>DANLTPDIRADIHAELVRLSFMPTRSESERYAIADRALAQYAALEILWHDNPDRTAQYQRIQVDHLGALLTRDRYKDVISHYQRLKKTGQIIPPWGQYWVASAYLKDHQPKKAQSIMTELFYHKETIAPDLSDEEL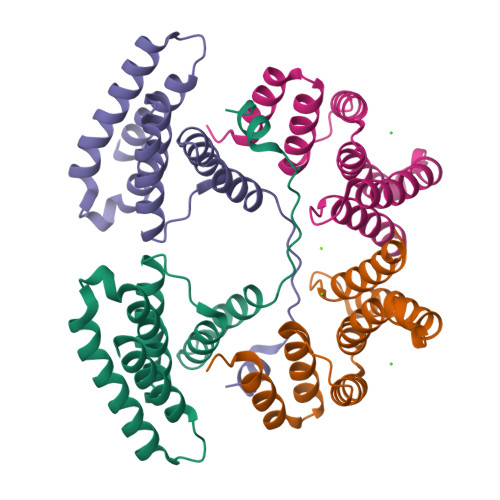ADLFYSHLESEN[2x]> AQSPATISLPQGGQFRLSISNTDPNMIFIPGDKVTAITAPGGMLADKRLTTAGGVLFTSVATRTFTIFVETALGQTFSVVATPVKGEGRVYRLMSAEPPSRPETRKWETAQAYEKLLISLNRAVLTGDIPDGYGEV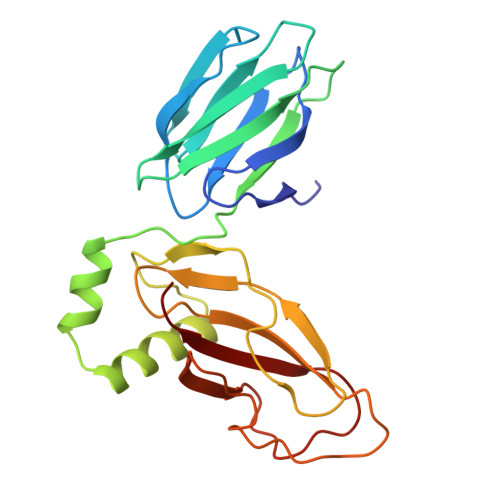KPLSDGIRLPGGFSVTPLKAWAGDQLRADRYELRNANTWGVALREQDFWKPGVRAVMFDNNAQTLMGGGRMTVTVIRGNG Our subsequent investigation of one gene cluster (Rv3093c-Rv3095) associated with ethionamide resistance that contained a putative monooxygenase/repressor pair with some resemblance to ethA/ethR, indicates that Rv3094c is likely a flavin-dependent monooxygenase that sulfoxygenates ethionamide, and Rv3095 is its transcriptional regulator. Ethionamide is a second-line anti-tubercular drug used to treat patients infected with multi-drug-resistant or extensively drug-resistant isolates, and is a pro-drug that requires metabolic activation before it can exert its cytotoxic effects. To investigate the mechanism of ethionamide sulfoxygenation by Rv3094c, we solved protein crystal structures of apo-Rv3094c, and Rv3094c in complex with FMN (Rv3094c-FMN) and ethionamide (Rv3094c-FMN-ETH), at resolutions of 1.91 Å, 2.00 Å, and 1.64 Å, respectively. All three crystals contained one tetramer per asymmetric unit, tetramers being formed by two homodimers, the C-terminal domain primarily mediating interactions between the two monomers.

The overall structure of the apo-Rv3094c monomer consists of an N-terminal domain (residues 7–95) composed of five α-helices, a middle domain (residues 96–214) composed of four α-helices and an eight-stranded β-barrel fold, and a C-terminal domain (residues 216–376), with a seven-helix bundle structure. The lack of a Rossmann fold suggests that Rv3049c can utilize either FAD or FMN, explaining the presence of FMN rather than FAD in the crystal structure obtained. A structure-based comparison between Rv3094c, one-component monooxygenases, two-component monooxygenases, and Baeyer-Villiger monooxygenases showed that Rv3094c clusters with two-component monooxygenases. Superposition of apo-Rv3094c structural homologs not only reveals strong structural conservation of overall topology, but confirms that the location of the FMN binding site, lying in the pocket between the β-sheet and the C-terminal domain, and stabilization of the flavin ring by hydrogen bonds are also conserved. Substrate binding, however, induces movements in the side chains of some amino acids in the apoenzyme and binary complex structures.

> VNQSETEIEILAEKIARWARARSAEIERDRRLPDELVTRLREAGLLRATMPREVAAPELAPGRALRCAEAVARGDASAGWCVSIAITSALLVAYLPARSREEMFGGGRGVAAGVWAPRGTARSVDGGVVVSGRWPFCSGINHADIMFAGCFVDDRQVPSVVALNKDELQVLDTWHTLGLRGTGSHDCVADDVFVPADRVFSVFDGPIVDRPLYRFPVFGFFALSIGAAALGNARAAIDDLVELAGGKKGLGSTRTLAERSATQAAAATAESALGAARALFYEVIEAAWQVSHDAEAVPVTMRNRLRLAATHAVRTSADVVRSMYDLAGGTAIYDNAPLQRRFRDAFTATAHFQVNEASRELPGRVLLDQPADVSML> MLMRPLDLTEKRGKKVTIYFEGKELEAYEGEKLPVALLANEIYWLTTSNEGRKRGAFTFGPVPMTVNGVKGLEARRIKVKDGMKIERQGYYDFHEEPVVEPGEIERVVVDVAIIGGGPAGIGAALELQQYLTVALIEERGWLGGDMWLKGIKQEGFNKDSRKVVEELVGKLNENTKIYLETSALGVFDKGEYFLVPVVRGDKLIEILAKRVVLATGAIDSTMLFENNDMPGVFRRDFALEVMNVWEVAPGRKVAVTGSKADEVIQELERWGIDYVHIPNVKRVEGNEKVERVIDMNNHEYKVDALIFADGRRPDINPITQAGGKLRFRRGYYSPVLDEYHRIKDGIYVAGSAVSIKPHYANYLEGKLVGAYILKEFGYDAQPCIYEEKLREYEPESLSIPRIPLDKFNLEDVQICGCDVSLKKVDEVIRKGITDLQIIKRLTHLAMGFCQGRYCLFNGAVVVSQRTGKKLSEIDLPVARSPIKNVKMGILARR;> MLPEKSEIVVIGGGIVGVTIAHELAKRGEEVTVIEKRFIGSGSTFRCGTGIRQQFNDEANVRVMKRSVELWKKYSEEYGFSFKQTGYLFLLYDDEEVKTFKRNIEIQNKFGVPTK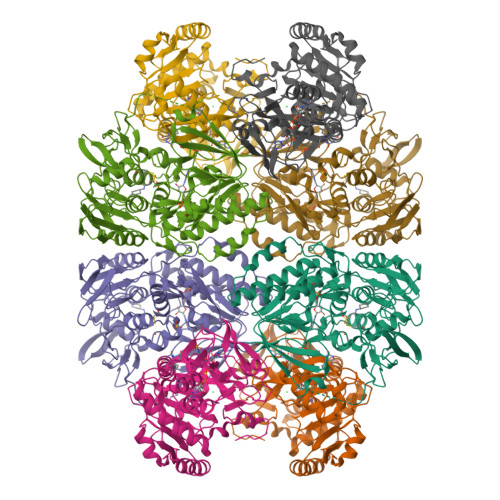LITPEEAKEIVPLLDISEVIAASWNPTDGKADPFEATTAFAVKAKEYGAKLLEYTEVKGFLIENNEIKGVKTNKGIIKTGIVVNATNAWANLINAMAGIKTKIPIEPYKHQAVITQPIKRGTINPMVISFKYGHAYLTQTFHGGIIGGIGYEIGPTYDLTPTYEFLREVSYYFTKIIPALKNLLILRTWAGYYAKTPDSNPAIGRIEELNDYYIAAGFSGHGFMMAPAVGEMVAELITKGKTKLPVEWYDPYRFERGELRTAALQMG Cytochrome cL (CytcL) is an essential protein in the process of methanol oxidation in methylotrophs. It receives an electron from the pyrroloquinoline quinone (PQQ) cofactor of methanol dehydrogenase (MDH) to produce formaldehyde. The two electrons are subsequently transferred from PQQ of MDH to the heme of cytochrome cL through an unknown mechanism, followed by its sequential transfer to CytcH, cytochrome c oxidase, and finally to ATP synthase in the cell membrane for the generation of ATP molecules. To help gain a better understanding of the mechanism, we determined the first crystal structure of heme c containing CytcL from the aquatic methylotrophic bacterium Methylophaga aminisulfidivorans MPT at 2.13 Å resolution.

The crystal contains four Ma-CytcL molecules in the asymmetric unit (ASU), in which the active sites (heme-binding pocket) from each subunit face each other. Although it appears to be a tetramer in the asymmetric unit, Ma-CytcL likely functions as a monomer in the cell. The structure of Ma-CytcL contains a typical cytochrome c fold consisting of six α-helices (α1-α6) and four 310 helices (η1-η4). Among the structural elements, four helices (α3, α4, α5, and η2), comprising the CXXCH motif, envelop the heme, as found in other cytochrome cL homologs. Each monomer of Ma-CytcL contains a heme cofactor covalently bound to the heme-binding region and coordinated by a metal ion, Fe(III) in heme. The iron atom is further coordinated by the axial ligands, including H92 and M132, as in typical cytochromes. Interestingly, three additional metal ions, Na+, Fe2+, and Ca2+, were also found in the subunit, with the Na+-binding site coinciding with the metal-binding sites in other structures. However, Ma-CytcL contains two Na+ ions (1Na+ and 2Na+) mainly surrounded by the loop between α3 and η2, in which a few residues form coordination bonds with the heme molecule. The Fe2+ binding site in Ma-CytcL is coordinated by typical metal-binding residues H94 and E97 and further stabilized by hydrogen bonds with a nearby water molecule (w11) (right).

>MTIKTFLPKKIRGIALLTVSVLSVVMIPVAQSQLVFRNTVTGDVLDLSFGKKGEKTEAVEHFLNTGENLYNTDDEAIKAGESLFMTACSGCHGHHAEGKLGPALGDDYYTYPKNANDKGLFETIYGGARSMMGPQYNNLTKDEILHIMAWVRSVYWGSADKADWLTEEQKANFKPAEVPEDFKEAMDNFNKTHH[4x]1-(4-iodophenyl)-3-[2-(4-sulfamoylphenyl)ethyl]urea 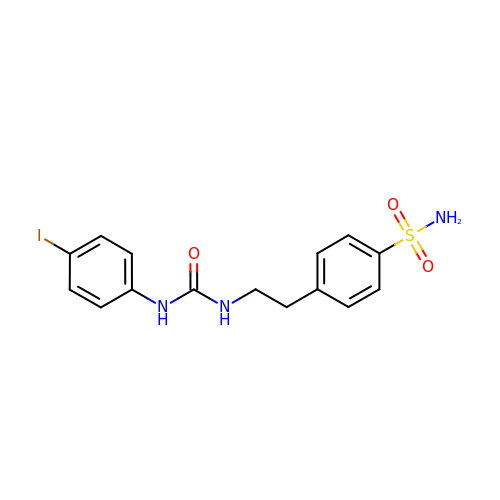| C15 H16 I N3 O3 S | YBQBJSKPHKMSDH-UHFFFAOYSA-N> MAHHHHHHSSGLEVLFQGPNEFETLELEH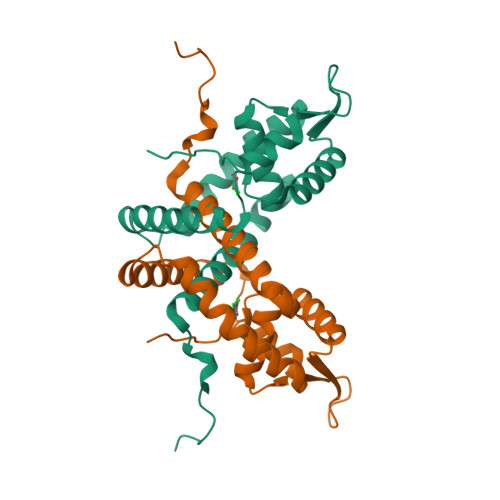LLWVNITQVKHSIERAWTRELKSLNLSTEKFAILHELMCLGGESTPHTLARRIVFEPHSVSAIVSRMEKDGLIIKTKDLDKKHMVRIKLSEKAIDTFYQALEISNRVYKQMMASITREEKVELSKTLTKLRNHTLPLTHKHTKTLTPFKYI> MRLLLFRQRNFRNLALEAYRPPPGLSALVGANAQGKTSLLLGIHLALGGEVPLGLADLVRFGEEEAWLHAEVETELGAYRLEHRLGPGGREVLLNGKRVSLRTLWELPGSVLVSPLDLEAVLGPKEERRAYLDRLIARFSRRYAALLSAYEKALRQRNALLKAGGEGLSAWDRELARYGDEIVALRRRFLRRFAPILREVHAALAAKEAGLRLEETAGEGVLRALEASRAEERERGQTLVGPHRDDLVFLLEGRPAHRFASRGEAKTLALALRLAEHRLLGEHHGEPPLLLVDEWGEELDEARRRAVLAYAQALPQAILAGLEAPP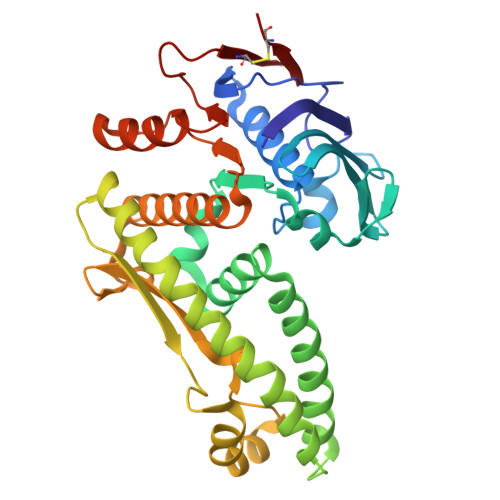GVPVCSVVRGVVLCPGA>[2x]GEGMWVPQQLPEIAGPLKKAGLKLSPQQISDLTGDPMGAVVALGGCTASFVSPNGLVVTNHHCAYGAIQLNSTAENNLIKNGFNAPTTADEVSAGPNARVFVLDEITDVTKDAKAAIAAAGDDALARTKALEAFEKKLIADCEAEAGFRCRLYSFSGGNTYRLFKNLEIKDVRLAYAPPGSVGKFGGDIDNWMWPRHTGDFAFYRAYVGKDGKPAAF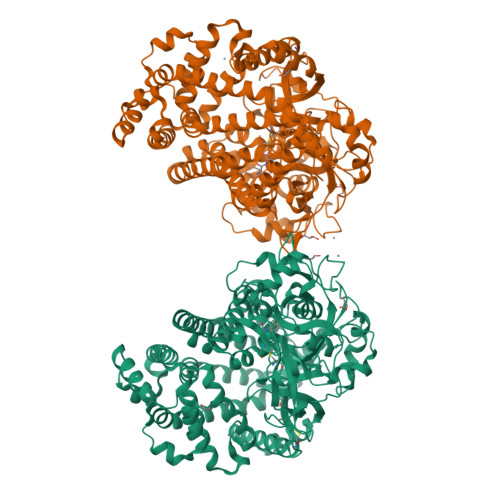SKDNVPYQPKHWLKFADQPLGAGDFVMVAGYPGSTNRYALAAEFDNTAQWTYPTIARHYKNQIAMVEAAGKQNADIQVKYAATMAGWNNTSKNYDGQLEGFKRIDAAGQKLREEAAVLGWLKGQGAKGQPALDAHAKLLDLLEQSKATRDRDLTLALFNNTAMLGSATQLYRLSIEREKPNAERESGYQERDLPAIEGGLKQLERRYVAAMDRQLQEYWLNEYIKLPADQRVAAVDAWLGGNDAAAVKRALDRLAGTKLGSTEERLKWFAADRKAFEASNDPAIQYAVAVMPTLLKLEQERKTRAGENLAARPVYLQALADYKKSQGEFVYPDANLSLRITFGNVMGYAPKDGMEYTPFTTLEGVVAKETGQDPFDSPKALLDAVAAKRYGGLEDKRIGSVPVNYLSDLDITGGNSGSPVLDAHGKLVGLAFDGNWESVSSNWVFDPKMTRMIAVDGRYLRWIMQEVYPAPQLLKEMNVGK>[2x]QQPLNEEFRPEMLQGKKVIVTGASKGIGREMAYHLAKM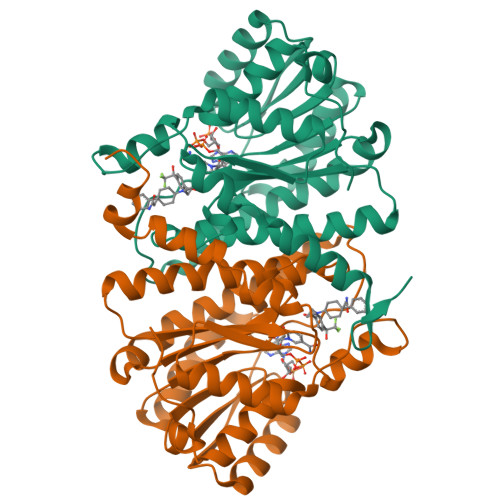GAHVVVTARSKETLQKVVSHCLELGAASAHYIAGTMEDMTFAEQFVAQAGKLMGGLDMLILNHITNTSLNLFHDDIHHVRKSMEVNFLSYVVLTVAALPMLKQSNGSIVVVSSLAGKVAYPMVAAYSASKFALDGFFSSIRKEYSVSRVNVSITLCVLGLIDTETAMKAVSGIVHMQAAPKEECALEIIKGGALRQEEVYYDSSLWTTLLIRNPSRKILEFLYSTSYNMDRFINK>[2x]VEYSRITKFFQEQPLEGYTLFSHRSAPNGFKVAIVLSELGFHYNTIFLDFNLGEHRAPEFVSVNPNARVPALIDHGMDNLSIWESGAILLHLVNKYYKETGNPLLWSDDLADQSQINAW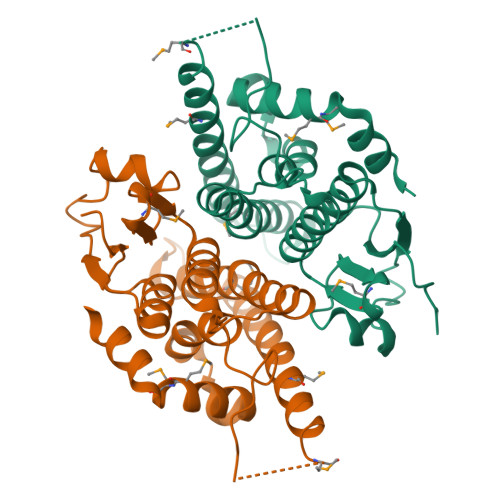LFFQTSGHAPMIGQALHFRYFHSQKIASAVERYTDEVRRVYGVVEMALAERREALVMELDTENAAAYSAGTTPMSQSRFFDYPVWLVGDKLTIADLAFVPWNNVVDRIGINIKIEFPEVYKWTKHMMRRPAVIKALRGE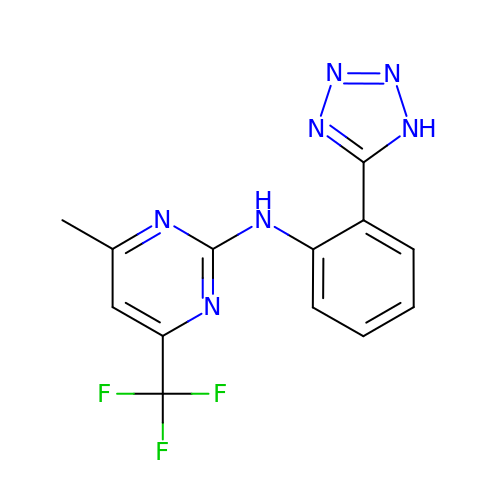4-methyl-N-[(2M)-2-(1H-tetrazol-5-yl)phenyl]-6-(trifluoromethyl)pyrimidin-2-amine | C13 H10 F3 N7 | XXKGCSWBGJTTJM-UHFFFAOYSA-N>[2x]MGSSHHHHHHSSGENLYFQGHMHYQKEEPSYFSHSPSPVEVYTEWDPLEEVIVGIMDDIRVPDWDKSLKAIIPEENHDFFQTYSGKRFPEELLIKARQEVETLAQILQAEGIRV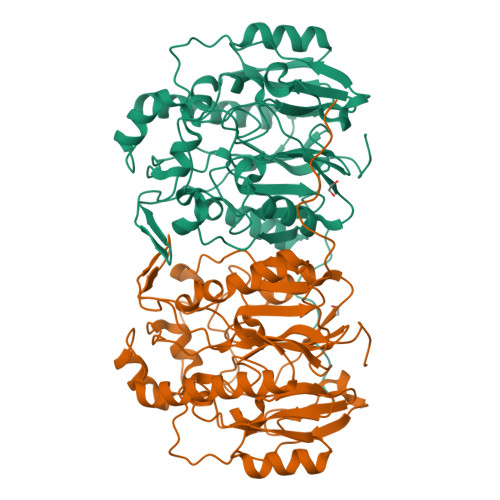KRPNESNHHQPIMTPHFTTGGTFYSAMPRDCLFAIGKKIIEVPMSWRSRYFETFAFRDILNDYFTRGAEWIAAPKPMLSDDVWEKDFDFEQEFPFRSIITEVEPLFDAADFMKMGRDIIGQRSHATNKKGIEWLRRTLGPDYHIHIYEFDEPAPMHIDTTILPLAPGRVLINKGWVPQIPDIFKDWEILNPPASNLPDDHPLYMSSNWIHTNVLMLDEKTVIVEEDEEALISAFRQWGFKTILCPFKHFQTFGGSFHCATLDVKRSGSLKSYI> GVFTFQDEYTSTIAPAKLYKALVTDADIIIPKAVETIQSVEIVEGNGGPGTIKKLTFIEGGESKYVLHKIEAIDEANLGYNYSIVGGVGLPDTIEKISFETKLVEGANGGSIGK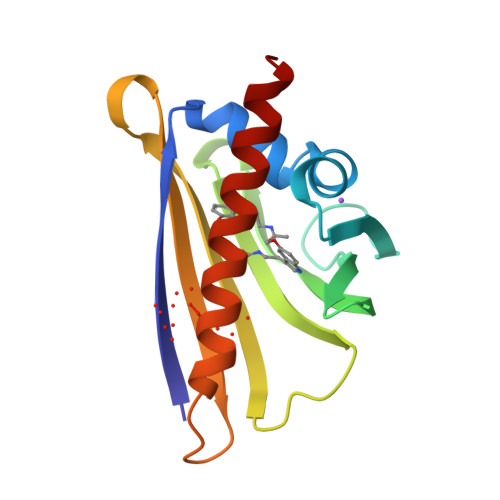VTIKIETKGDAQPNEEEGKAAKARGDAFFKAIESYLSAHPD Recently, the AAA+ ATPase TRIP13 has been shown to collaborate with p31comet to promote MCC disassembly and checkpoint inactivation. p31comet acts as an adaptor to recruit C-Mad2 to TRIP13. TRIP13 then induces the conformational change of C-Mad2 to O-Mad2 in a process that requires ATP hydrolysis. We have determined the crystal structure of human TRIP13 in its ADP-bound state, and identified TRIP13 residues critical for p31comet–Mad2 binding and for coupling ATP hydrolysis to Mad2 unfolding. In conclusion, using a combination of biophysical and biochemical approaches, we have demonstrated that TRIP13–p31comet catalyzes the conversion of C-Mad2 to O-Mad2 without the global unfolding of Mad2.

We subjected human TRIP13 E253A mutant (which was deficient in ATP hydrolysis) bound to ATP and the p31comet–Mad2 complex to crystallization, and obtained diffracting crystals. Structure determination, however, revealed that the crystals contained TRIP13 alone in the ADP-bound state. Even though the ATPase-deficient mutant of TRIP13 was used in our studies, the residual ATPase activity of TRIP13 E253A presumably converted ATP to ADP, and contributed to the dissociation of the complex. Structure of human TRIP13 bound to ADP is highly similar to that of the C. elegans PCH-2 promoter bound to ADP, with an RMSD of 1.57 Å for all atoms. Both contain an N-terminal domain (NTD), a large AAA+ subdomain, and a small AAA+ subdomain. ADP is bound at the interface between the large and small AAA+ subdomains. The only discernable difference is located at the so-called pore loop. This region forms a helix in PCH-2, but does not have visible electron density and is likely flexible in human TRIP13. Because the human TRIP13 structure does not form a closed hexamer and has a disordered pore loop, we used the structure of the C. elegans PCH-2 hexamer to guide our subsequent mutagenesis and biochemical studies. TRIP13 G320 is located at the hinge between its large and small AAA+ subdomains.

> MDEAVGDLKQALPCVAESPTVHVEVHQRGSSTAKKEDINLSVRKLLNRHNIVFGDYTWTEFDEPFLTRNVQSVSIIDTELKVKDSQPIDLSACTVALHIFQLNEDGPSSENLEEETENIIAANHWVLPAAEFHGLWDSLVYDVEVKSHLLDYVMTTLLFSDKNVNSNLITWNRVVLLHGPPGTGKTSLCKALAQKLTIRLSSRYRYGQLIEINSHSLFSKWFSESGKLVTKMFQKIQDLIDDKDALVFVLIDAVESLTAARNACRAGTEPSDAIRVVNAVLTQIDQIKRHSNVVILTTSNITEKIDVAFVDRADIKQYIGPPSAAAIFKIYLSCLEELMKCQIIYPRQQLLTLRELEMIGFIENNVSKLSLLLNDISRKSEGLSGRVLRKLPFLAHALYVQAPTVTIEGFLQALSLAVDKQFEERKKLAAYI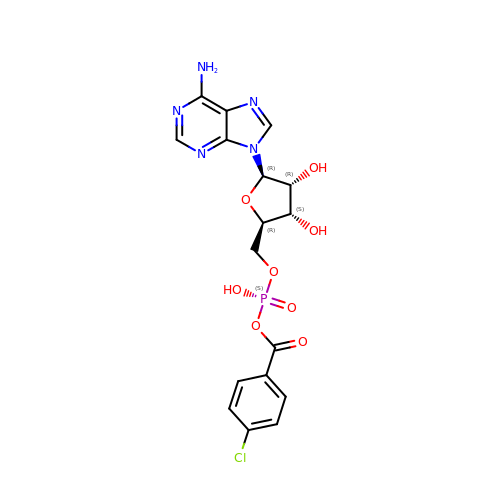5'-O-[(S)-{[(4-chlorophenyl)carbonyl]oxy}(hydroxy)phosphoryl]adenosine | C17 H17 Cl N5 O8 P | RVDNKWBGRIIRML-XNIJJKJLSA-N> MAGMKTSPSQDEEACVLAIQLATSTVLPMILKSAIELDILNTISKAGPGNYLSPSDLASKLLMSNPHAPIMLERILRVLATYKVLGCKPSELSDGEVEWLYCWTPVCKFLSNNEDGASIAPLLLVHQDQVPMKSWYHLTDAILDGGTAFNKAYGMNIFDYASQDPQFNKVFNRSMAGHSTITMKKILETYNGFEGLKSIVDVGGGSGATLNMIISKYPTIKGINFDLPHVVGDSPIHPGVE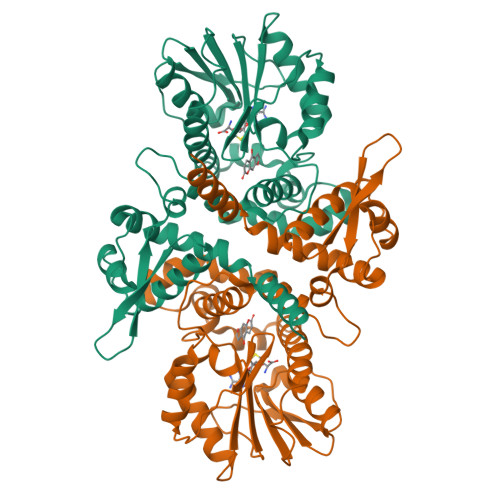HVGGDMFASVPKGDAIFLKWIFHSWSDEDCLRILKNCYEALADNKKVIVAEFIIPEVPGGSDDATKSVVHLDAVMLAYVPGGKERTEKEFEALATSAGFKSFRKVCCAFNTWIMEFSK N-benzyladenosine | 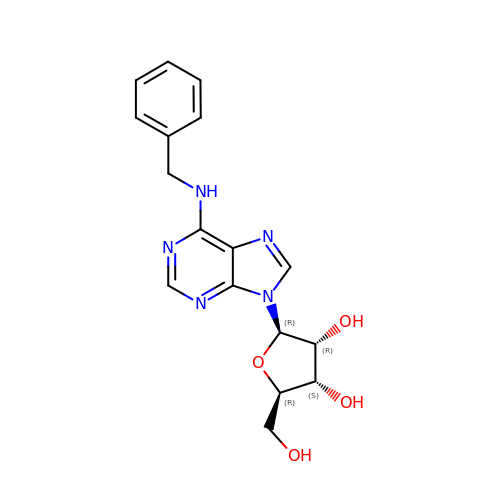C17 H19 N5 O4 | MRPKNNSABYPGBF-LSCFUAHRSA-N>[2x]AECSVDIQGNDQMQFNTNAITVDKSCKQFTVNLSHPGNLPKNVMGHNWVLSTAADMQ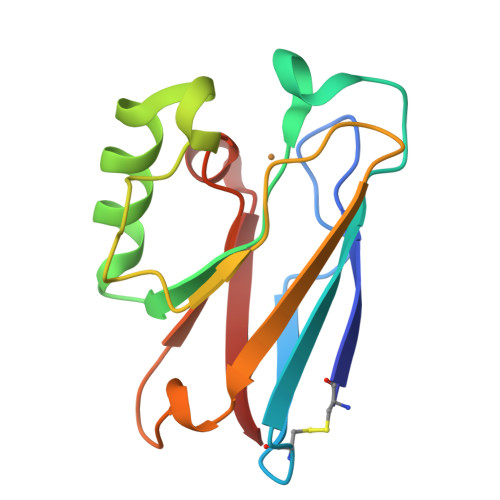GVVTDGMASGLDKDYLKPDDSRVIAHTKLIGSGEKDSVTFDVSKLKEGEQYMFFCSPHQGAGMKGTLTLK> MYSDQTYEVIKNRTLENINLDIYKGEGSFLNNMVSGNNLELSKIYLELSKMHKMAFIQDTYNQFLDKRVNEFGVYRKLGTESNGEVEFIGEKGTVINNGTIISYRDLLFVVIKDVTIGSEEGDNSPVQALEVGKKYNLPTNCEFKLVDNISGVTKITNTRSFEGGTDIETDEELKERFYKIQRNQATSGNKAHYEEWALEVDGVYNVKVYPRWDGPGTVKVLIFGKNNQAVDTETIERCQQHIDEEKPIGPTITVVTPLPIEISISAVMKLEDGYTLDNVKESFLESINTYFRDIRGEIIYTKVMGILINTTGVHDLSNLLINGS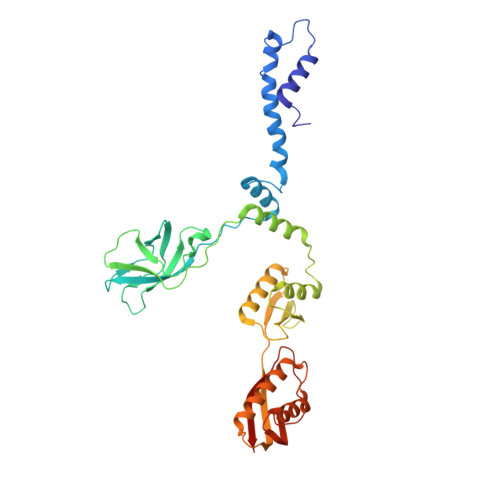TDNITINEDKIPSVTTVNFSEVENQ> METFDPTELPELLKLYYRRLFPYSQYYRWLNYGGVIKNYFQHREFSFTLKDDIYIRYQSFNNQSDLEKEMQKMNPYKIDIGAVYSHRPNQHNTVKLGAFQAQEKELVFDIDMTDYDDVRRCCSSADICPKCWTLMTMAIRIIDRALKEDFGFKHRLWVYSGRRGVHCWVCDESVRKLSSAVRSGIVEYLSLVKGGQDVKKKVHLSEKIHPFIRKSINIIKKYFEEYALVNQDILENKESWDKILALVPETIHDELQQSFQKSHNSLQRWEHLKKVASRYQNNIKNDKYGPWLEWEIMLQYCFPRLDINVSKGINHLLKSPFSVHPKTGRISVPIDLQKVDQFDPFTVPTISFICRELDAISTNEEEKEENEAESDVKHRTRDYKKTSLAPYVKVFEHFLENLDKSRKGELLKKSDLQKDF;> GGSMEFSGRKWRKLRLAGDQRNASYPHCLQFYLQPPSENISLIEFENLAIDRVKLLKSVENLGVSYVKGTEQYQSKLESELRKLKFSYRENLEDEYEPRRRDHISHFILRLAYCQSEELRRWFIQQEMDLLRFRFSILPKDKIQDFLKDSQLQFEAISDEEKTLREQEIVASSPSLSGLKLGFESIYKIPFADALDLFRGRKVYLEDGFAYVPLKDIVAIILNEFRAKLSKALALTARSLPAVQSDERLQPLLNHLSHSYTGQDYSTQGNVGKISLDQIDLLSTKSFPPCMRQLHKALRENHHLRHGGRMQYGLFLKGIGLTLEQALQFWKQEFIKGKMDPDKFDKGYSYNIRHSFGKEGKRTDYTPFSCLKIILSNPPSQGDYHGCPFRHSDPELLKQKLQSYKISPGGISQILDLVKGTHYQVACQKYFEMIHNVDDCGFSLNHPNQFFCESQRILNGGKDIKKEPIQPETPQPKPSVQKTKDASSALASLNSSLEMDMEGLEDYFSEDS;> GPGSADEEQVFHFYWLDAYEDQYNQPGVVFLFGKVWIESAETHVSCCVMVKNIERTLYFLPREMKIDLNTGKETGTPISMKDVYEEFDEKIATKYKIMKFKSKPVEKNYAFEIPDVPEKSEYLEVKYSAEMPQLPQDLKGETFSHVFGTNTSSLELFLMNRKIKGPCWLEVKSPQLLNQPVSWCKVEAMALKPDLVNVIKDVSPPPLVVMAFSMKTMQNAKNHQNEIIAMAALVHHSFALDKAAPKPPFQSHFCVVSKPKDCIFPYAFKEVIEKKNVKVEVAATERTLLGFFLAKVHKIDPDIIVGHNIYGFELEVLLQRINVCKAPHWSKIGRLKRSNMPKLGGRSGFGERNATCGRMICDVEISAKELIRCKSYHLSELVQQILKTERVVIPMENIQNMYSESSQLLYLLEHTWKDAKFILQIMCELNVLPLALQITNIAGNIMSRTLMGGRSERNEFLLLHAFYENNYIVPDKQIFRKPQQKLGDEDEEIDGDTNKYKKGRKKAAYAGGLVLDPKVGFYDKFILLLDFNSLYPSIIQEFNICFTTVQRVASEAQKVTEDGEQEQIPELPDPSLEMGILPREIRKLVERRKQVKQLMKQQDLNPDLILQYDIRQKALKLTANSMYGCLGFSYSRFYAKPLAALVTYKGREILMHTKEMVQKMNLEVIYGDTDSIMINTNSTNLEEVFKLGNKVKSEVNKLYKLLEIDIDGVFKSLLLLKKKKYAALVVEPTSDGNYVTKQELKGLDIVRRDWCDLAKDTGNFVIGQILSDQSRDTIVENIQKRLIEIGENVLNGSVPVSQFEINKALTKDPQDYPDKKSLPHVHVALWINSQGGRKVKAGDTVSYVICQDGSNLTASQRAYAPEQLQKQDNLTIDTQYYLAQQIHPVVARICEPIDGIDAVLIATWLGLDPTQFRVHHYHKDEENDALLGGPAQLTDEEKYRDCERFKCPCPTCGTENIYDNVFDGSGTDMEPSLYRCSNIDCKASPLTFTVQLSNKLIMDIRRFIKKYYDGWLICEEPTCRNRTRHLPLQFSRTGPLCPACMKATLQPEYSDKSLYTQLCFYRYIFDAECALEKLTTDHEKDKLKKQFFTPKVLQDYRKLKNTAEQFLSRSGYSEVNLSKLFAGCAVKS;> MSASAQQLAEELQIFGLDCEEALIEKLVELCVQYGQNEEGMVGELIAFCTSTHKVGLTSEILNSFEHEFLSKRLSKARHSTCKDSGHAGARDIVSIQELIEVEEEEEILLNSYTTPSKGSQKRAISTPETPLTKRSVSTRSPHQLLSPSSFSPSATPSQKYNSRSNRGEVVTSFGLAQGVSWSGRGGAGNISLKVLGCPEALTGSYKSMFQKLPDIREVLTCKIEELGSELKEHYKIEAFTPLLAPAQEPVTLLGQIGCDSNGKLNNKSVILEGDREHSSGAQIPVDLSELKEYSLFPGQVVIMEGINTTGRKLVATKLYEGVPLPFYQPTEEDADFEQSMVLVACGPYTTSDSITYDPLLDLIAVINHDRPDVCILFGPFLDAKHEQVENCLLTSPFEDIFKQCLRTIIEGTRSSGSHLVFVPSLRDVHHEPVYPQPPFSYSDLSREDKKQVQFVSEPCSLSINGVIFGLTSTDLLFHLGAEEISSSSGTSDRFSRILKHILTQRSYYPLYPPQEDMAIDYESFYVYAQLPVTPDVLIIPSELRYFVKDVLGCVCVNPGRLTKGQVGGTFARLYLRRPAADGAERQSPCIAVQVVRI;> GPGSMAAGRAQVPSSEQAWLEDAQVFIQKTLCPAVKEPNVQLTPLVIDCVKTVWLSQGRNQGSTLPLSYSFVSVQDLKTHQRLPCCSHLSWSSSAYQAWAQEAGPNGNPLPREQLLLLGTLTDLSADLEQECRNGSLYVRDNTGVLSCELIDLDLSWLGHLFLFPRWSYLPPARWNSSGEGHLELWDAPVPVFPLTISPGPVTPIPVLYPESASCLLRLRNKLRGVQRNLAGSLVRLSALVKSKQKAYFILSLGRSHPAVTHVSIIVQVPAQLVWHRALRPGTAYVLTELRVSKIRGQRQHVWMTSQSSRLLLLKPECVQELELELEGPLLEADPKPLPMPSNSEDKKDPESLVRYSRLLSYSGAVTGVLNEPAGLYELDGQLGLCLAYQQFRGLRRVMRPGVCLQLQDVHLLQSVGGGTRRPVLAPCLRGAVLLQSFSRQKPGAHSSRQAYGASLYEQLVWERQLGLPLYLWATKALEELACKLCPHVLRHHQFLQHSSPGSPSLGLQLLAPTLDLLAPPGSPVRNAHNEILEEPHHCPLQKYTRLQTPSSFPTLATLKEEGQRKAWASFDPKALLPLPEASYLPSCQLNRRLAWSWLCLLPSAFCPAQVLLGVLVASSHKGCLQLRDQSGSLPCLLLAKHSQPLSDPRLIGCLVRAERFQLIVERDVRSSFPSWKELSMPGFIQKQQARVYVQFFLADALILPVPRPCLHSATPSTPQTDPTGPEGPHLGQSRLFLLCHKEALMKRNFCVPPGASPEVPKPALSFYVLGSWLGGTQRKEGTGWGLPEPQGNDDNDQKVHLIFFGSSVRWFEFLHPGQVYRLIAPGPATPMLFEKDGSSCISRRPLELAGCASCLTVQDNWTLELESSQDIQDVLDANKSLPESSLTDLLSDNFTDSLVSFSAEILSRTLCEPLVASLWMKLGNTGAMRRCVKLTVALETAECEFPPHLDVYIEDPHLPPSLGLLPGARVHFSQLEKRVSRSHNVYCCFRSSTYVQVLSFPPETTISIPLPHIYLAELLQGGQSPFQATASCHIVSVFSLQLFWVCAYCTSICRQGKCTRLGSTCPTQTAISQAIIRLLVEDGTAEAVVTCRNHHVAAALGLCPREWASLLDFVQVPGRVVLQFAGPGAQLESSARVDEPMTMFLWTLCTSPSVLRPIVLSFELERKPSKIVPLEPPRLQRFQCGELPFLTHVNPRLRLSCLSIRESEYSSSLGILASSC;> MQPGSSRCEEETPSLLWGLDPVFLAFAKLYIRDILDMKESRQVPGVFLYNGHPIKQVDVLGTVIGVRERDAFYSYGVDDSTGVINCICWKKLNTESVSAAPSAARELSLTSQLKKLQETIEQKTKIEIGDTIRVRGSIRTYREEREIHATTYYKVDDPVWNIQIARMLELPTIYRKVYDQPFHSSALEKEEALSNPGALDLPSLTSLLSEKAKEFLMENRVQSFYQQELEMVESLLSLANQPVIHSASSDQVNFKKDTTSKAIHSIFKNAIQLLQEKGLVFQKDDGFDNLYYVTREDKDLHRKIHRIIQQDCQKPNHMEKGCHFLHILACARLSIRPGLSEAVLQQVLELLEDQSDIVSTMEHYYTAF;> MMLPKPGTYYLPWEVSAGQVPDGSTLRTFGRLCLYDMIQSRVTLMAQHGSDQHQVLVCTKLVEPFHAQVGSLYIVLGELQHQQDRGSVV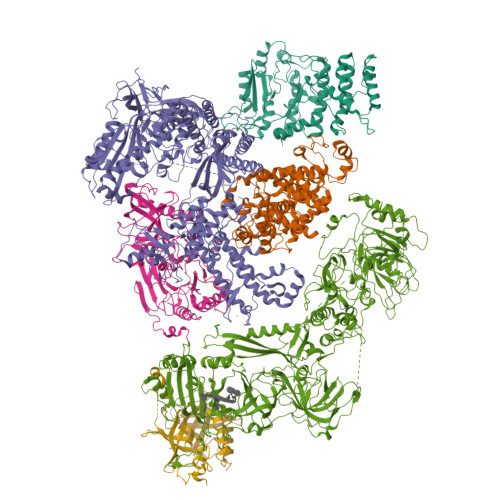KARVLTCVEGMNLPLLEQAIREQRLYKQERGGSQ> GSHMSKSLKKLVEESREKNQPEVDMSDRGISNMLDVNGLFTLSHITQLVLSHNKLTMVPPNIAELKNLEVLNFFNNQIEELPTQISSLQKLKHLNLGMNRLNTLPRGFGSLPALEVLDLTYNNLSENSLPGNFFYLTTLRALYLSDNDFEILPPDIGKLTKLQILSLRDNDLISLPKEIGELTQLKELHIQGNRLTVLPPELGNLDLTGQKQVFKAENNPWVTPIADQFQLGVSHVFEYIRSETYKYLYGRHMQANPEPPKKNNDKSKKISRKPLAAKNR;> GSPEGVPICGACRRPIEGRVVNAMGKQWHVEHFVCAKCEKPFLGHRHYERKGLAYCETHYNQLFGDVCFHCNRVIEGDVVSALNKAWCVNCFACSTCNTKLTLKNKFVEFDMKPVCKKCYEKFPLELKKRLKKLAETLGRK

Ras suppressor-1 (Rsu-1) is a leucine-rich repeat (LRR)-containing protein that is crucial for regulating cell adhesion and is involved in such physiological and pathological processes as focal adhesion assembly and tumor metastasis. Rsu-1 interacts with zinc-finger type multi-LIM domain-containing adaptor protein PINCH-1, known to be involved in the integrin-mediated consensus adhesome, but not with its highly homologous family member PINCH-2. Rsu-1 does not have catalytic activity but its primary sequence analysis indicates a leucine-rich repeat (LRR)-containing protein that implicates for protein-binding functions. We also showed that Rsu-1 can be assembled, via PINCH-1-binding, into a heteropentamer complex comprising Rsu-1, PINCH-1, ILK, Parvin, and Kindlin-2, which constitute a major consensus integrin adhesome crucial for focal adhesion assembly.

Our structural results reveal that Rsu-1 folds into a rigid arc-shaped architecture with eight consecutive LRRs shielded by two terminal capping modules, and it engages via its extensive conserved concave surface the LIM5 domain of PINCH-1 in a pattern analogous to some LRR–protein ligand complex formation that is referred to as “hand-clasp”. The superposition of the structure of Rsu-1 bound form with that of its unbound form showed an RMSD of 0.56-Å for the 249 Cα atom pairs, indicating that Rsu-1 retains its rigid architecture, and does not undergo major structural change upon the binding to PINCH-1. The conformation in the C-terminal region of Rsu-1, which is disordered in the unbound form, essentially remains the same structural arrangement as the unbound form, suggesting that the C-terminal region is not involved in the direct binding to PINCH-1. The binding interface is relatively extensive and continuous and buries approximately 2321 Å2 of solvent-accessible surface area that is comparable to those found in the LRR-protein ligand complexes at high affinity. The analysis of electrostatic surface potential of the Rsu-1-LIM complex reveals that each protein surface displays distinct complementary charge distributions and binding architecture at the interface. Two polar residues of Arg165 and Asp166 from the seventh LRR motif of Rsu-1 that are highly conserved across species play a prominent role in the interface, by forming salt bridges with Asp295 and Arg314 of PINCH-1 LIM5 domain, respectively. In addition to the hydrogen bonds and salt bridges, a hydrophobic residue of Phe71 of Rsu-1 that contacts to Phe307 and Thr280 in the PINCH-1 LIM5 domain also significantly contributes to the binding interaction. Our data revealed that the calculated melting temperature (Tm) of Rsu-1 bound to PINCH-1 LIM5 domain (Tm = 67.7 ± 0.5 °C) was significantly higher (11.6 °C) than that in the absence of the protein ligand (Tm = 56.1 ± 0.2 °C), suggesting a significant preference of the interaction for the increased protein stability.> LVHVASVEKGRSYEDFQKVYNAIALKLREDDEYDNYIGYGPVLVRLAWHISGTWDKHDNTGGSYGGTYRFKKEFNDPSNAGLQNGFKFLEPIHKEFPWISSGDLFSLGGVTAVQEMQGPKIPWRCGRVDTPEDTTPDNGRLPDADKDAGYVRTFFQRLNMNDREVVALMGAHALGKTHLKNSGYEGPQGAANNVFTNEFYLNLLNEDWKLEKNDANNEQWDSKSGYMMLPTDYSLIQDPKYLSIVKE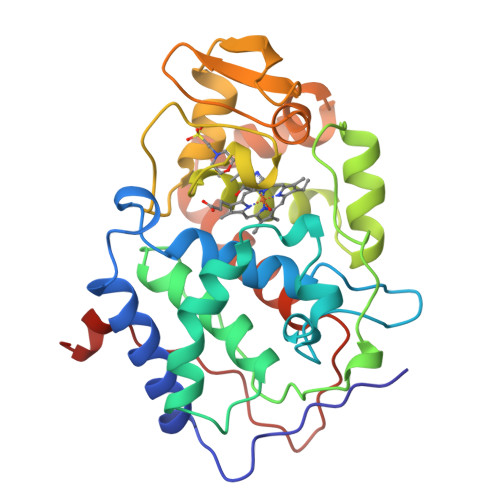YANDQDKFFKDFSKAFEKLLEDGITFPKDAPSPFIFKTLEEQGL(R)-reticuline | C19 H23 N O4 | 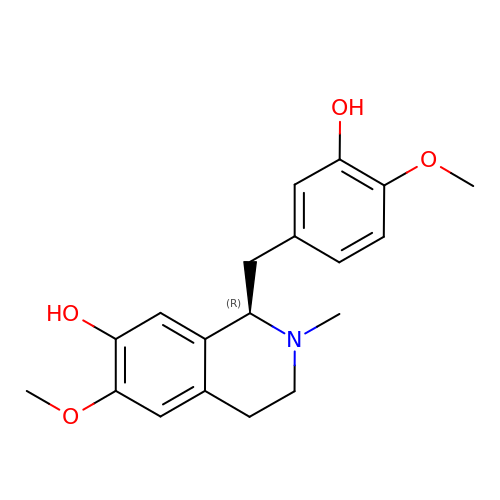BHLYRWXGMIUIHG-UHFFFAOYSA-N> LAFNEPLNIVSHLNDDWFLFGDARSDCTYVENNGHPKLDWLDLDPKLCNSGRISAKSGNSLFRSFHFTDFYNYSGEGDQVIFYEGVNFSPSHGFKCLANGDNKIWMGNKARFYARLYEKMAQYRSLSIVTVSYAYGGNAKPTSICKDNKLTLNNPTFISKESNYADYYYVSEANFTLQGCDEFIVPLCVFNGHSRGSSSDPANTYYMDSQMYYNTVTGVFYGFNSTLDVGTTVQNPGLDLTCSYLALSPGNYKAVSLEFLLSLPSKAICLLKPKRFMPVQVVDSRWNSTRQSDNMTAVACQLPYCFFR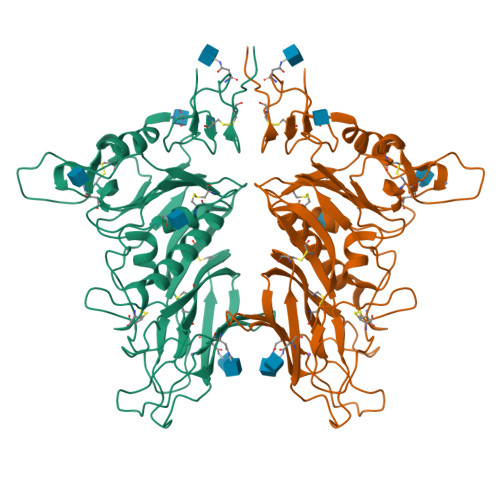NTSADYSGDTHDVHHGDLYFRQLLSGLLYNVSCIAQQGAFLYNNVSSIWPVYGYGHCPTAANIGYMAPICLYDSDPLVPR> GAMDYSLVKALQTAQQNFVISDPSIPDNPIVYASQGFLTLTGYALSEVLGRNCRFLQGPETDPKAVEKVRKGLERGEDTTVVLLNYRKDGSTFWNQLFIAALRDGEGNVVNYLG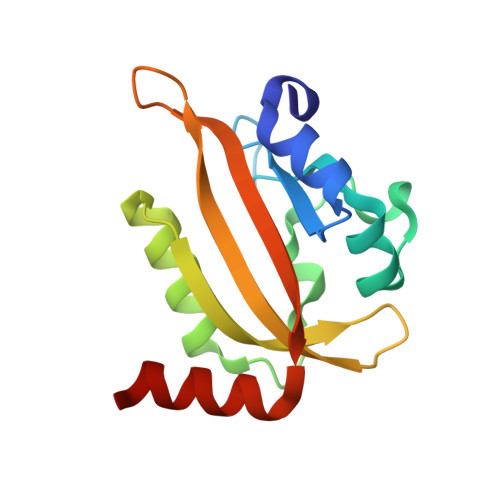VQCKVSEDYAKAFLKNEEKE> GGCVQVDRYEDVVKAPAPAGLAGFWQTKGPQSAMMSPDAIASLIVTKEGDTFDCRQWQRVIAQPGKLMNR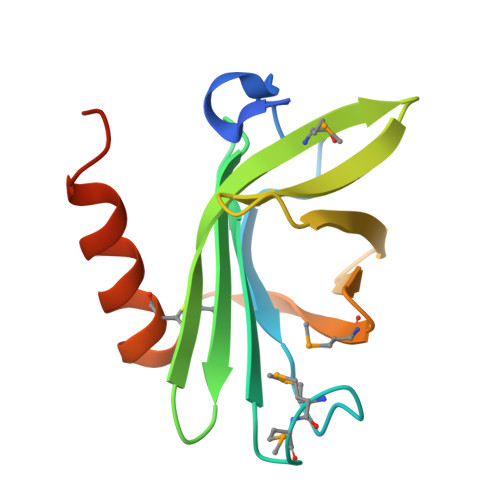DSEIYNVTASLDIYPVEREGNTISYDRMTLSRVERLTPECEKAWAKARATGPVSAPASTR> SNAMSTISRDSCPALRAGVRLQHDRARDQWVLLAPERVVELDDIALVVAQRY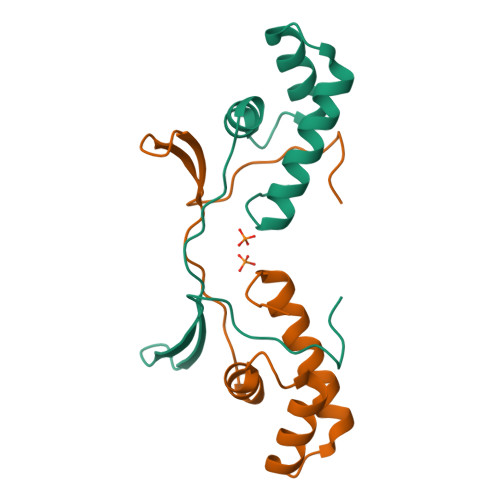DGTQSLAQIAQTLAAEFDADASEIETDVIELTTTLHQKRLLRL>GHMDSPEIRELEKFANEFKVRRIKLGYTQTNVGEALAAVHGSEFSQTTICRFENLQLSFKNACKLKAILSKWLEEAEQVGALYNEKVGANERKRKRRTTISIAAKDALERHFGEQNKPSSQEIMRMAEELNLEKEVVRV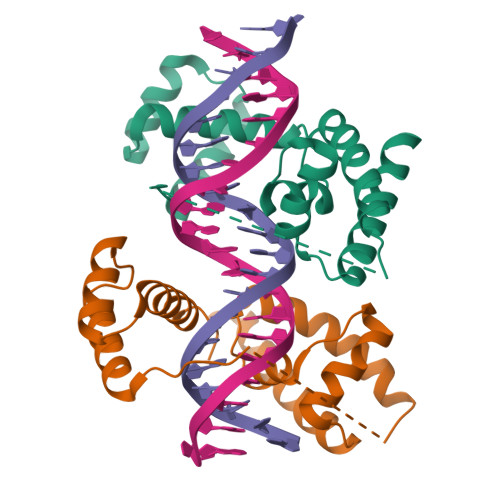WFCNRRQREKRVK[4x]>GSHNMAEMVETVCGPVPVEQLGKTLIHEHFLFGYPGFQGDVTRGTFRED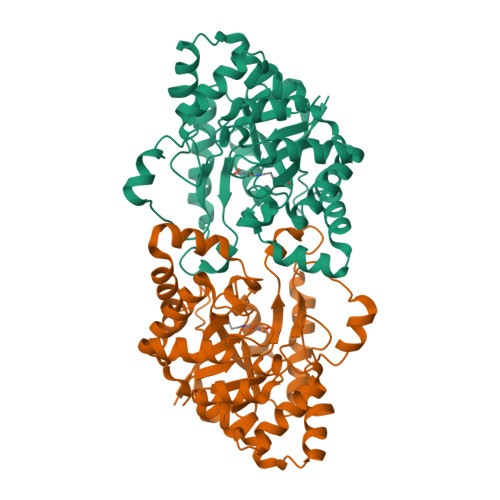ESLRVAVEAAEKMKRHGIQTVVDPTPNDCGRNPAFLRRVAEETGLNIICATGYYYEGEGAPPYFQFRRLLGTAEDDIYDMFMAELTEGIADTGIKAGVIKLASSKGRITEYEKMFFRAAARAQKETGAVIITHTQEGTMGPEQAAYLLEHGADPKKIVIGHMCGNTDPDYHRKTLAYGVYIAFDDFGIQGMVGAPTDEERVRTLLALLRDGYEKQIMLSHDTVNVWLGRPFTLPEPFAEMMKNWHVEHLFVNIIPALKNEGIRDEVLEQMFIGNPAALFSA[2x]> MAVKVEYDLKRLRNIGIAAHIDAGKTTTTERILYYTGRIHKIGEVHEGAATMDFMEQERERGITITAAVTTCFWKDHRINIIDTPGHVDFTIEVERSMRVLDGAIVVFDSSQGVEPQSETVWRQAEKYKVPRIAFANKMDKTGADLWLVIRTMQERLGARPVVMQLPIGREDTFSGIIDVLRMKAYTYGNDLGTDIREIPIPEEYLDQAREYHEKLVEVAADFDENIMLKYLEGEEPTEEELVAAIRKGTIDLKITPVFLGSALKNKGVQLLLDAVVDYL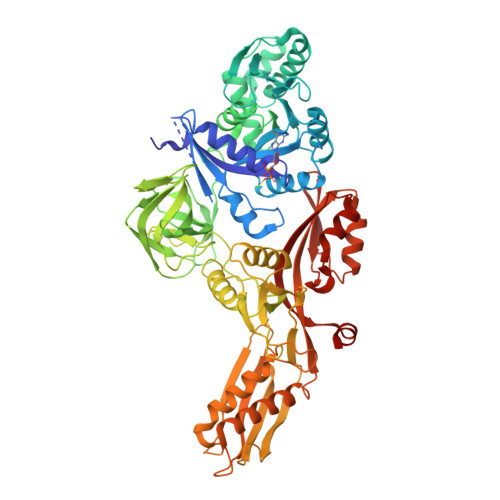PSPLDIPPIKGTTPEGEVVEIHPDPNGPLAALAFKIMADPYVGRLTFIRVYSGTLTSGSYVYNTTKGRKERVARLLRMHANHREEVEELKAGDLGAVVGLKETITGDTLVGEDAPRVILESIEVPEPVIDVAIEPKTKADQEKLSQALARLAEEDPTFRVSTHPETGQTIISGMGELHLEIIVDRLKREFKVDANVGKPQVAYRETITKPVDVEGKFIRQTGGRGQYGHVKIKVEPLPRGSGFEFVNAIVGGVIPKEYIPAVQKGIEEAMQSGPLIGFPVVDIKVTLYDGSYKEVDSSEMAFKIAGSMAIKEAVQKGDPVILEPIMRVEVTTPEEYMGDVIGDLNARRGQILGMEPRGNAQVIRAFVPLAEMFGYATDLRSKTQGRGSFVMFFDHYQEVPKQVQEKLIKGQ> EPCCDSCRCT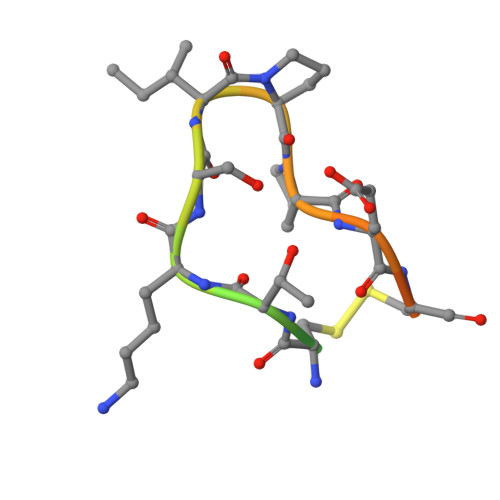KSIPPECHCANI(2S)-4-[{[(2S,3S,4R,5R)-5-(6-amino-9H-purin-9-yl)-3,4-dihydroxytetrahydrofuran-2-yl]methyl}(carboxylatomethyl)sulfonio]-2-ammoniobutanoate 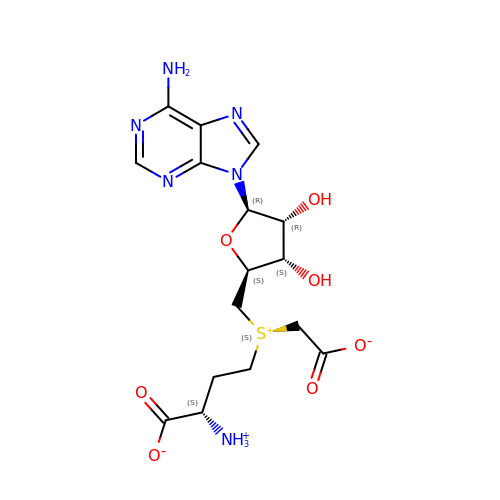| C16 H22 N6 O7 S | VFFTYSZNZJBRBG-HEOPWLPUSA-N> MNILIFGPNGSGKGTQGNL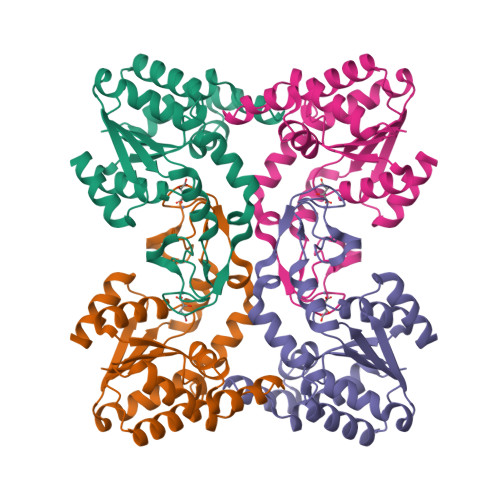VKDKYSLAHIESGGIFREHIGGGTELGKKAKEFIDRGDLVPDDITIPMVLETLESKGKDGWLLDGFPRNTVQAQKLFEALQEKGMKINFVIEILLPREVAKNRIMGRRICKNNPNHPNNIFIDAIKPNGDVCRVCGGALSARADDQDEGAINKRHDIYYNTVDGTLAAAYYYKNMAAKEGFVYIELDGEGSIDSIKDTLLAQLA The anti-apoptotic (pro-survival) proteins of the BCL-2 family include BCL-2, BCL-XL, MCL-1, BCL-w and BFL-1/A1. These proteins bind to and sequester the apoptosis effectors, as well as the apoptosis sensitizers, BIM, BID, PUMA, NOXA, BAD, BMF, HRK and BIK5,6. An elongated hydrophobic groove is thus formed along the surface of BCL-2 and BCL-XL proteins, spanning approximately 20 Å to serve as the binding site for the amphipathic α-helical BH3 domains of their pro-apoptotic partners. Herein we present cyclic peptides (CPs) with nanomolar-level binding affinities to BCL-2 or BCL-XL, and further reveal the structural and functional mechanisms of how these CPs target two proteins in a fashion that is remarkably different from traditional small-molecule inhibitors.

Since the overall structures and surface grooves of BCL-2 and BCL-XL proteins are highly similar we wanted to know whether cp1 can also bind to BCL-XL and whether it exhibits a preference between two proteins. To understand the beneath structural basis for this selectivity of cp1, we co-crystalized and determined the complex structures of cp1 bound to BCL-2 and BCL-XL proteins with high resolutions at 2.1 Å and 2.0 Å, respectively. In both structures, the electron densities for cp1 were well defined. It is not very surprising that like the small-molecule inhibitors and BH3-mimetic peptides, cp1 also binds to the hydrophobic surfaces (formed by α2, α4, α5, α8 helices) of BCL-2 or BCL-XL where the BH3-only proteins usually bind. Interestingly, the conformation of cp1 is almost identical in these two different complexes. In addition, the overall conformations of BCL-2 and BCL-XL bound by cp1 are also very similar, as indicated by the RMSD of only 0.26 Å for all their Cα atoms. Taking a closer look, we analyzed in detail the key amino-acid residues within 5 Å around cp1 in two complex structures to seek for differences, and found that most of these residues are conserved in BCL-2 and BCL-XL, except for two pairs of residues (i.e. D111, M115 in BCL-2 and corresponding A104, L108 in BCL-XL). However, in BCL-XL, the corresponding residue is A104, which has a shorter side chain and can’t directly interact with cp1-G6. However, in the BCL-XL-cp1 complex, there is some unfilled space between cp1-G6 and A104 of BCL-XL, potentially causing a weaker interaction at this position. However, upon cp1 binding, the overall conformation of α3 and α4 helices of BCL-2/BCL-XL remains roughly the same as in the crystal structure of ligand-free BCL-XL, still exhibiting a flat interaction surface similar to the unbound state. The respective SASAs in the structures of BCL-2-BAX, BCL-2-venetoclax, BCL-2-cp1 are 979 Å2, 1007 Å2, 768 Å2, while in those of BCL-XL-BID, BCL-XL-ABT-737, BCL-XL-cp1 are 1135 Å2, 1061 Å2, 828 Å2, implying relatively smaller SASA values upon cp1 binding for both BCL-2 and BCL-XL.

> MSQSNRELVVDFLSYKLSQKGYSWSQFMAAVKQALREAGDEFELRYRRAFSDLTSQLHITPGTAYQSFEQVVNELFRDGVNWGRIVAFFSFGGALCVESVDKEMQVLVSRIAAWMATYLNDHLEPWIQENGGWDTFVELYG;> CPARYGWDYECX>GPGSLTVYQGANATNYQQYKKKGVQFDDLLAINSDVMAWLTVKGTHIDYPIVQGENNLEYINKSVEGEYSLSGSVFLDYRNKVTFEDKYSLIYAHHMAGNVMFGELPNFRKKSFFNKHKEFSIETKTKQKLKINIFACIQTDAFDSLLFNPIDVDISSKNEFLNHIKQKSVQYREILTTNESRFVALSTCEDMTTDGRIIVIGQIE[2x]

Here, we focus on Spy0129, an accessory sortase responsible for assembly of the covalent polymeric shaft of the pili expressed by Streptococcus pyogenes (group A streptococcus; GAS) serotype M1. Spy0129 is the only pilus-specific sortase of GAS M1, having been shown by gene knockout to be essential for the polymerization of Spy0128. In this process, Spy0129 cleaves between Thr and Gly of the sortase-recognition motif EVPTG of Spy0128, and links the Thr carboxylate via an isopeptide bond to the ε-amino group of Lys161 of the next major pilin subunit. The overall structure of Spy0129 conforms to the archetypal sortase fold, in which a highly-twisted, 8-stranded β-sheet folds over to generate a core β-barrel, whose surface is decorated with loops and helices.

The Spy0129 structure solved in this study comprises the complete 237-residue polypeptide, with the exception of the first 35 residues, which constitute the transmembrane anchor and were omitted from the construct (Spy012936–237) to permit soluble expression. Spy0129 was crystallized in the space group I4122, with two molecules in the asymmetric unit. Crystals could only be obtained in the presence of 0.2 M Zn2+ and the asymmetric unit was found to contain 19 bound Zn2+ ions, which were used to derive initial phases by single wavelength anomalous diffraction (SAD) methods. The structure was subsequently refined at 2.3 Å resolution (R = 20.4%, Rfree = 26.0%; see Table 1 for full details). The most distinctive features of the Spy0129 structure, however, are the three long connecting loops β2/β3 (residues 86–105), β4/β5 (residues 126–150) and β6/β7 (residues 173–214), which between them shape the presumed substrate-binding region. Distinct differences are seen in the active sites of the two independent Spy0129 molecules in the crystal. Alternative positions of these loops are stabilised by bound zinc ions that coordinate the active site residues in different ways in the two molecules, and by crystal packing. Structural superpositions, however, show that in molecule B of Spy0129 the conformations of β4 and the β4/β5 loop match the equivalent structures of all other sortases, and that His126 superimposes on the catalytic histidine in each case. In this molecule, His126 is directed towards Cys221, with a bound zinc ion bridging between Cys221 Sγ and His126 Nδ1, whereas His127 projects into solution. We conclude that the bound Zn2+ ions in the crystal structure are probably not of functional importance, although they do play a role in stabilising alternate conformations of several loops and in stabilising the crystal packing.>[2x]MGLWFEEGAEERQVLGPFREFLKAEVAPGAAERDRTGAFPWDLVRKLAEFGVFGALVPEAYGGAGLSTRLFARMVEAIAYYDGALALTVASHNSLATGHILLAGSEAQKEAFLPKLASGEALGAW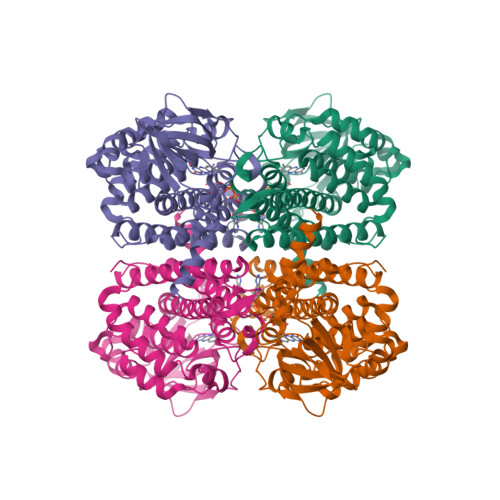GLTEPGSGSDAAALKTKAEKVEGGWRLNGTKQFITQGSVAGVYVVMARTDPPPSPERKHQGISAFAFFRPERGLKVGRKEEKLGLTASDTAQLILEDLFVPEEALLGERGKGFYDVLRVLDGGRIGIAAMAVGLGQAALDYALAYAKGREAFGRPIAEFEGVSFKLAEAATELEAARLLYLKAAELKDAGRPFTLEAAQAKLFASEAAVKACDEAIQILGGYGYVKDYPVERYWRDARLTRIGEGTSEILKLVIARRLLEAV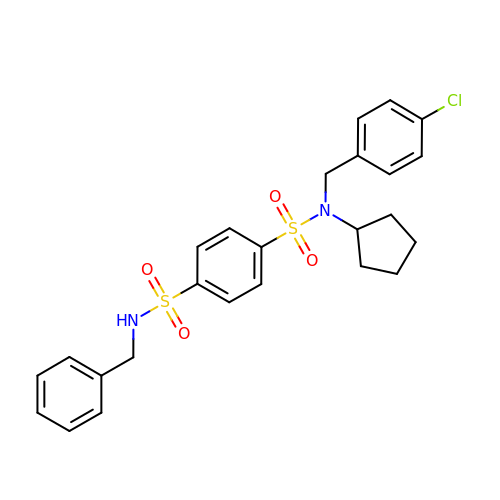~{N}1-[(4-chlorophenyl)methyl]-~{N}1-cyclopentyl-~{N}4-(phenylmethyl)benzene-1,4-disulfonamide | C25 H27 Cl N2 O4 S2 | CWMNFAGFCBOHSI-UHFFFAOYSA-N>[2x]MKFSKGIHAIDSHTMGEPTRIVVGGIPQINGETMADKKKYLEDNLDYVRTALMHEPRGHNDMFGSIITSSNNKEADFGIIFMDGGGYLNMCGHGSIGAATVAVETGMVEMVEPVTNINMEAPAGLIKAKVMVENEK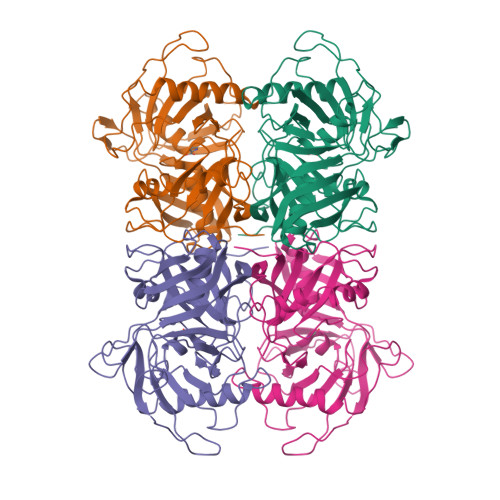VKEVSITNVPSFLYMEDAKLEVPSLNKTITFDISFGGSFFAIIHAKELGVKVETSQVDVLKKLGIEIRDLINEKIKVQHPELEHIKTVDLVEIYDEPSNPEATYKNVVIFGQGQVDRSPCGTGTSAKLATLYKKGHLKIDEKFVYESITGTMFKGRVLEETKVGEFDAIIPEITGGAYITGFNHFVIDPEDPLKYGFTVLEHHHHHH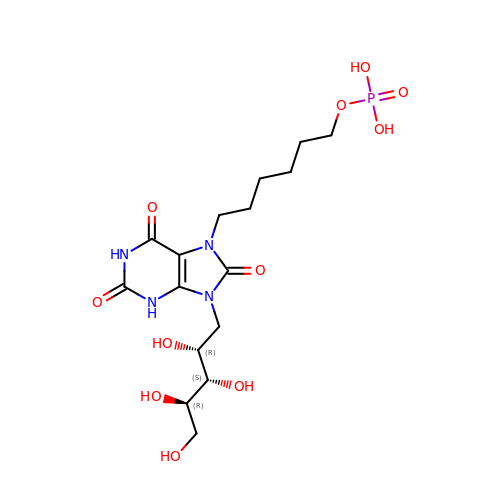3-(1,3,7-TRIHYDRO-9-D-RIBITYL-2,6,8-PURINETRIONE-7-YL ) HEXANE 1-PHOSPHATE | C16 H27 N4 O11 P | SLRQIPDGMUYATQ-FOGDFJRCSA-N>MIPTIDLEEVSDKILNQKIREASERWGCFRVINHGVSLSLMAEMKKTVIDLFQRPYEVKVRNTDVLLGSGYRAPNEINPYYEALGLYDMASPHAVNTFCDQLEASADQREIMVKYAKAINGLATDLARKLAESYGLVETDFFKEWPSQFRINKYHFKPE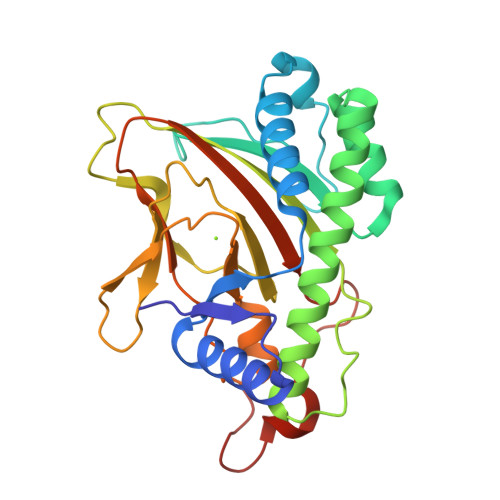TVGKLGVQLHTDSGFLTILQDDENVGGLEAMDNSSGTFFPIDPLPNTLAINLGDMATIWSNGRLCNVKHRVQCKEATMRYSIASFLLGPMDTDLEPPSEFVDAEHPRLYKP[3x]> MGSSHHHHHHSSGRENLYFQGHMVARLLEEHGFETKTNVIVQGNCVEQEIDVVAERDGERYMIECKFHNIPVYTGLKEAMYTYARFLDVEKHGFTQPWIFTNTKFSEEAKKYAGCVGIKLTGWSYPEKEGIEVLLESK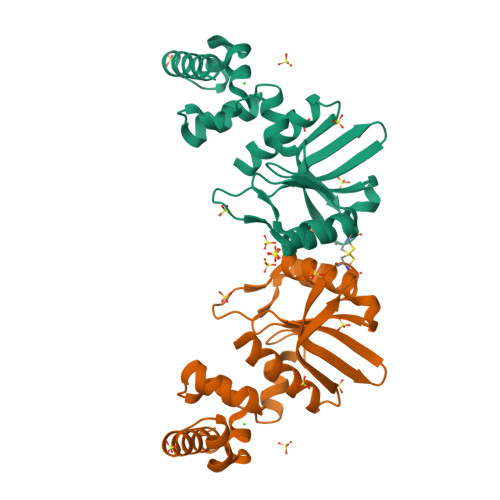GLYPITILRIDKEVLDELVRAGLVFCRDVVSAGEEKLREIGLSAKKAREVIAEAKKVIGGS(4S)-8-{2-[3-oxo-3-(pyrrolidin-1-yl)propoxy]phenoxy}indolizine-2-carbonitrile 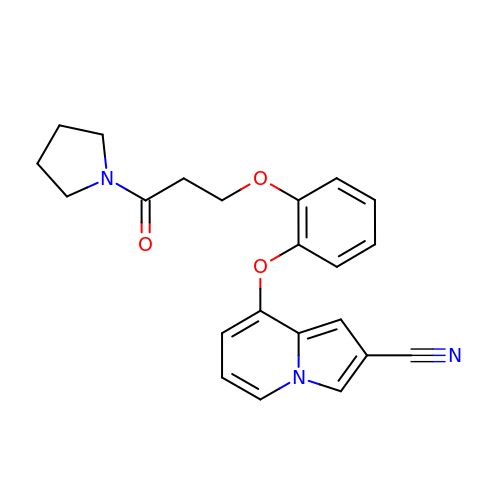| C22 H21 N3 O3 | PEIZFCTZWSLJCB-UHFFFAOYSA-N> GAEHDGLTGLLNRNSLQMRLAAAIDRVEASGESLAVICIDLDHFKEANDQHGHLAGDALLVETARRLQSAVQAPSFAARLGGDEFIVVQIAGGDQPAVAAELAGRLIEMLAAPVPFD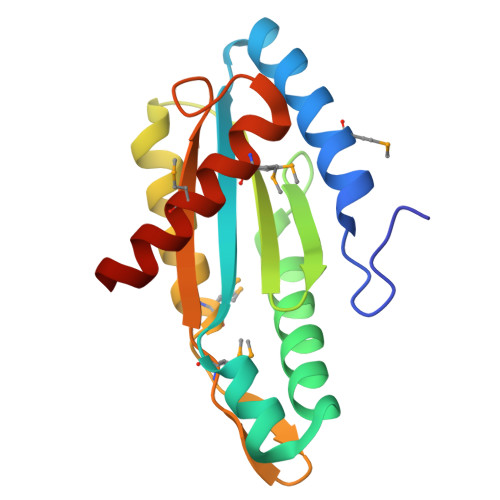GQELAMGSSLGVSLYPDDGRTAEALMANADMALYRAKESGR(4S)-3-BENZYL-6-CHLORO-2-METHYL-4-PHENYL-3,4-DIHYDROQUINAZOLINE 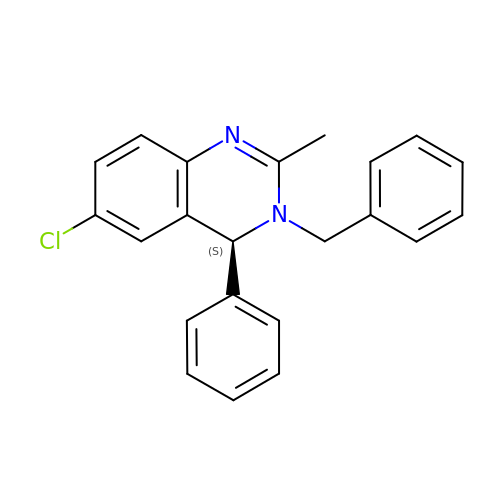| C22 H19 Cl N2 | HYYQDTGAVFYWEW-QFIPXVFZSA-N> HHHHHHMILCCGEALIDMLPRETTGGETAFQPFAGGSVFNTAIALGRLGVPTGFFSGISSDFFGDVLRDTLARSNVDYSFAAISNRPTTLAFVRLVDGQARYAFYDENTAGRML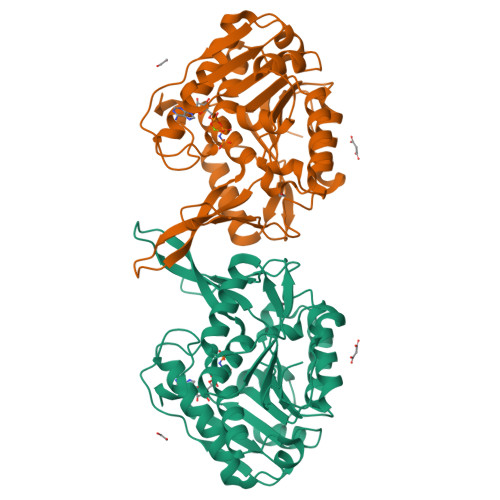SRNDMPYVDETISAMLFGCISLISEPCGSVYETLLAREAPNRVMFLDPNIRANLITVRKTHLTRMKRMIALADIVKLSDEDLDWFGEKGSHDEIAAEWLKLGPKLVVITKGAHGAVAYTNHATVPVPGVKVDVVDTVGAGDTVNAGILASLHSQGLLTKDALANLSEDQIHSAVALGVRAAAVTVSRAGANPPWAHEM> MKKQNDIPQPIRGDKGATVKIPRNIERDRQNPDMLVPP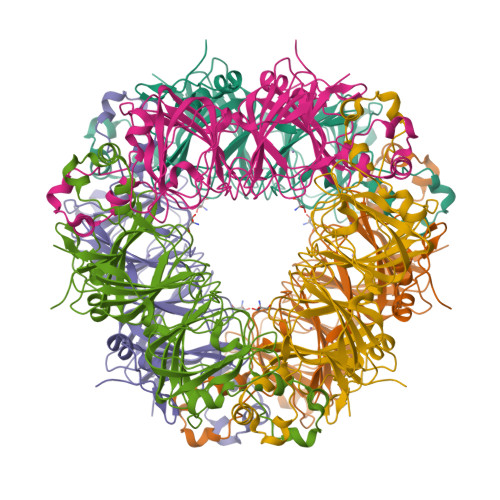ETDHGTVSNMKFSFSDTHNRLEKGGYAREVTVRELPISENLASVNMRLKPGAIRELHWHKEAEWAYMIYGSARVTIVDEKGRSFIDDVGEGDLWYFPSGLPHSIQALEEGAEFLLVFDDGSFSENSTFQLTDWLAHTPKEVIAANFGVTKEEISNLPGKEKYIFENQLPGSLKDDIVEGPNGEVPYPFTYRLLEQEPIESEGGKVYIADSTNFKVSKTIASALVTVEPGAMRELHWHPNTHEWQYYISGKARMTVFASDGHARTFNYQAGDVGYVPFAMGHYVENIGDEPLVFLEIFKDDHYADVSLNQWLAMLPETFVQAHLDLGKDFTDVLSKEKHPVVKKKCSK>[2x]MSAKDTADLSPLLEANRKWADECAAKDSTYFSKVAGSQAP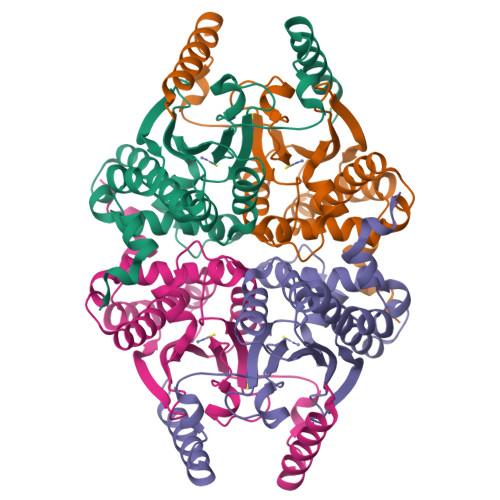EYLYIGCADSRVSPAQLFNMAPGEVFVQRNVGNLVSNKDLNCMSCLEYTVDHLKIKHILVCGHYNCGACKAGLVWHPKTAGVTNLWISDVREVRDKNAAKLHGLSADDAWDKMVELNVEAQVFNVCASPIVQAAWARGQPLSVHGIVYTPGTGLVKELIKPITGMEDAGALLRADLKQHCFFSESLA[({4-[4-(cyclopropyloxy)phenyl]pyridin-2-yl}amino)methanediyl]bis(phosphonic acid) | C15 H18 N2 O7 P2 | 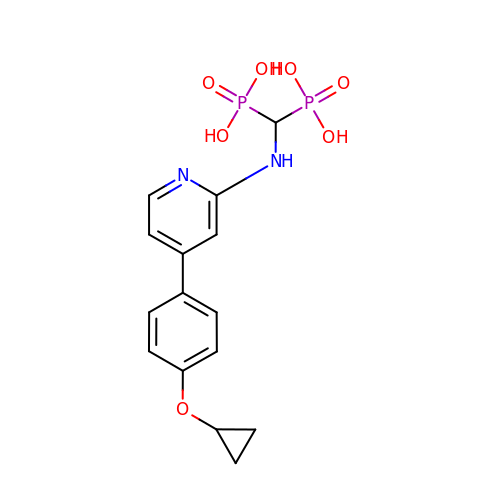MYPRZOLXSMRMEV-UHFFFAOYSA-N> FQRYMEIVIVVDHSMVKKYNGDSDSIKAWVYEMINTITESYSYLKIDISLSGLEIWSGKDLIDVEASAGNTLKSFGEWRAKDLIHRISHDNAQLLTATDFDGATIGLAYVASMCNPKRSVGVIQDHSSVNRLVAITLAHEMAHNLGVSHDEGSCS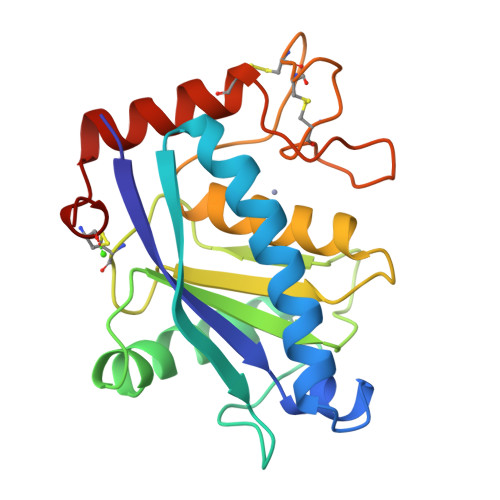CGGKSCIMSPSISDETIKYFSDCSYIQCRDYISKENPPCILN Among the SMC complexes, cohesin establishes cohesion between replicated sister chromatids, which forms the basis for faithful chromosome segregation during cell division. A characteristic feature of cohesin is its ability to bind DNA by topological embrace, which underpins sister chromatid cohesion (Haering et al., 2008). The cohesin ring consists of three core components: two SMCs and a kleisin subunit. Mis4Scc2/NIPBL is known as the cohesin loader.

We assembled cohesin onto a linear 125-bp dsDNA substrate in the presence of Mis4-Ssl3 and ADP·BeF3– and separated the gripping reaction by sucrose gradient centrifugation. We visualized this cohesin loading intermediate by cryo-electron microscopy (cryo-EM) at an average resolution of 3.9 Å. The model covers the Psm1 head and proximal coiled coil bound to the Rad21 C terminus, the Psm3 head and neck bound by the Rad21 N-terminal domain, as well as Mis4 and 32 bp of DNA. The DNA lies on top of the engaged ATPase heads, which are nucleotide bound and in a configuration competent for ATP hydrolysis. Mis4 clamps the DNA onto the ATPase heads, making widespread contacts with Psm1 and Psm3. The U-shaped Mis4 hook binds the engaged Psm1-Psm3 ATPase heads, whereas the Mis4 N-terminal handle contacts the Psm3 neck region. Mis4 and Psm3 together form a protein ring that topologically encircles the DNA. The lumen of the ring is lined with positive charges mainly clustered on the Mis4 surface. Although the U-shaped Mis4 hook can be superimposed with a root-mean-square deviation (RMSD) of only 1.0 Å, the angle at which the N-terminal handle emerges is tilted by 40°. The cryo-EM map was of sufficient quality to build amino acids 5–12 of the Rad21 N-tail, forming a loop wedged between the Psm3 ATPase head and the DNA.

> MGRLLRLEVENFKSYRGHQIIGPFEDFTSIIGPNGAGKSNLMDAISFVLGVKSSHLRSTNVKELIYRGKILQRDNTDFTDSSNPTTAYVKLMYELDNGEQREYKRAITPSGATEYKIDEEIVTFSEYCGSLQKENILVRARNFLVFQGDVETIASQSPLELSKLVEQISGSLEYKSEYDKSKDEQDKAVNLSAHSFNKKRGINAELRQYQEQKTEAERYQSQKEKRDSAQLVYLLWKLFHLEKSISSNMAEVTRLKADSIQLIERRDENTKEIEKLKEKEGSIRRNLLAFDRKVRKQEKLIASKRPELISIAEKALESKSNLRKIQRKAAEIEKDYSDQASTLQVLENQLTSLSAAEKEFLKDMQEKEQLKGLRLLPEDKEEYEGLRSEADKLNSNLLFKLQTLNRNIKVTSQSKDSLTSIVGDLESKIKSLHESVSSLDTERADLLAKINEKIESLELEKHDQQKKRLTYSELFHKTQELNEELQSCLQKILEASADRNESKQDAKKREALYALKRIYPEVKGRIIDLCTPTQKKYESAIAAALGKNFDAIVVETQAVAKECIDYIKEQRIGIMTFFPMDTIAASPVNQKFRGTHKGARLAIDVLNFESEYERVMISAVGNTLICDSMTVARDLSYNKRLNAKTVTLEGTVIHKTGLITGGSSNNRSAKHWDDHDFDLLTQTKDRLMHQIGEIEYQKSSCVITESDTVKLHSLESEISLLKDKYTVVSRSVEDKKKEIGHYESLIKEKQPHLSELEMELRNFVKSRDELQIQVEKVEEKIFSGFCKRIGISDIHTYDEIHRTFTQSFTQKQLEFTKQKSLLENRISFEKQRVSDTRLRLERMHKFIEKDQESIDNYEQNREALESEVATAEAELELLKEDFASENSKTEKILLAASEKKLVGKRLVSELTKLSGNITLLESEIDRYVSEWHAILRKCKLEDIDVPLREGSLTSIPIDDVSNSGDITMGEEPSEPVINFEKFGVEVDYDELDEELRNDGSESMASVLQEKLREYSEELDQMSPNLRAIERLETVETRLAKLDEEFAAARKAAKNAKERFNAVKQKRLQKFQAAFSHISEQIDPIYKELTKSPAFPLGGTAYLTLDDLDEPYLGGIKFHAMPPMKRFRDMDQLSGGEKTMAALALLFAIHSYQPSPFFVLDEIDAALDQTNVTKIANYIRQHASSGFQFVVISLKNQLFSKSEALVGIYRDQQENSSRTLSINLEGYVE;> MFYSEAILSKKGPLAKVWLAAHWEKKLSKVQTLHTSIEQSVHAIVTEETAPMALRLSGQLMLGVVRIYSRKARYLLEDCTEALMRLKMSFQPGQVDMIEPATALQSLKGKDAVTQSANLTLPETITEFDLLVPDSTFDFQWSQLLRTPSRSSNTLELHSLPISSSPSFPSSQLSIEAGRNAQVESGFSLGESFAHVGNDMQFHLPISNSGAATPRSVHSDNQSQISIEVGRDAPAAAATDLSGIIGPQMTKSPASSVTHFSTPSMLPIGGTSLDDELLAPVDDLNLDLGLDDLLGDEQGANAPAIEADEQAETSSIHLPSDIMEDDSSRPAAAGVEEGQVVESATAPQQEKINPQKTVRRQRAIIDPVTELSSKQMKKQLADTSSITSPLCLNTSSIVFNATVNFTRNGKFNTSIFSSNLNPKVNELLQADFKQAILRKRKNESPEEVEPAKHQRTDTSTENQETAEVLDPEEIAAAELANITEAAIATLPQETVVQPEGEAPELGSPMGFPVTALESADDSLFDAPPVMLDEADLLGSERLDSSVSEALPSSQTAKDSLRNKWDPYTEGEKVSFQTLSAGCNREEAVQLFFDVLVLATKDVISVKQDVAIQNEITLTAKRGMLLSSL;> MYITKIVIQGFKSYKDYTVIEPLSPHHNVIVGRNGSGKSNFFAAIRFVLSDAYTHLSREERQALLHEGPGATVMSAYVEVTFANADNRFPTGKSEVVLRRTIGLKKDEYSLDKKTVSKTEVINLLESAGFSRSNPYYIVPQGRVTSLTNAKDSERLELLKEVAGTQIYENRRAESNKIMDETIQKSEKIDELLQYIEERLRELEEEKNDLAVYHKKDNERRCLEYAIYSREHDEINSVLDALEQDRIAALERNDDDSGAFIQREERIERIKAEITELNHSLELLRVEKQQNDEDYTNIMKSKVALELQSSQLSRQIEFSKKDESSKLNILSELESKISEKENELSEILPKYNAIVSEADDLNKRIMLLKNQKQSLLDKQSRTSQFTTKKERDEWIRNQLLQINRNINSTKENSDYLKTEYDEMENELKAKLSRKKEIEISLESQGDRMSQLLANITSINERKENLTDKRKSLWREEAKLKSSIENVKDDLSRSEKALGTTMDRNTSNGIRAVKDIAERLKLEGYYGPLCELFKVDNRFKVAVEATAGNSLFHIVVDNDETATQILDVIYKENAGRVTFMPLNKLRPKAVTYPDASDALPLIQYLEFDPKFDAAIKQVFSKTIVCPSIETASQYARSHQLNGITLSGDRSDKKGALTAGYRDYRNSRLDAIKNVKTYQIKFSDLQESLEKCRSEIESFDQKITACLDDLQKAQLSLKQFERDHIPLKDELVTITGETTDLQESMHHKSRMLELVVLELHTLEQQANDLKSELSSEMDELDPKDVEALKSLSGQIENLSHEFDAIIKERAHIEARKTALEYELNTNLYLRRNPLKAEIGSDNRIDESELNSVKRSLLKYENKLQIIKSSSSGLEEQMQRINSEISDKRNELESLEELQHEVATRIEQDAKINERNAAKRSLLLARKKECNEKIKSLGVLPEEAFIKYVSTSSNAIVKKLHKINEALKDYGSVNKKAYEQFNNFTKQRDSLLARREELRRSQESISELTTVLDQRKDEAIERTFKQVAKSFSEIFVKLVPAGRGELVMNRRSELSQSIEQDISMDIDTPSQKSSIDNYTGISIRVSFNSKDDEQLNINQLSGGQKSLCALTLIFAIQRCDPAPFNILDECDANLDAQYRSAIAAMVKEMSKTSQFICTTFRPEMVKVADNFYGVMFNHKVSTVESISKEEAMAFVEG;> MLFEMTPETFKKVNSSNRIIKGLQYTPLASSIPLENGLQNVLYPSSKFQNEPLQLNSEESSIMQRYVDMLNPGATFVNDSETFNFYKNALSAMITEPAMPAMRVNASPVLDQKVCNSDSLSELNDFTKSLIQPSMLMCEPKEKPDASSINTNRSSSDNGFLTPSSSPRSPSCSRVFNAVQLCSPKKSKDDITTPKKRLMEDTYSPRESPSKIQRLQDVLLKQLQDTRLLISQVIEAENSEDFSSNSLFIKREDDDGKHISSHAIEKLYMALTKLSRLGACDKLLEEGSIILVKQILEKELKELPVACYSIINLHDSLTQFPNLDFILKTTALVLFIIFLVPSFKKLQNEESILHLLNILHSIFEYTVPEAIDNIVQSKTSDARTSEIQHLSVLLQKVANVLNILSKVAHEIPLSEAVVIRIVYLFPKVSTLDNSFKTKLPNCNSSSFDFLKAPLFQTLQYLFRLYPYQRDFIIEESLTNFSHLPTARSVSRTYRLSNGKSIQYYSTLFVRLIQSCSIQNLFDSEIVQSESKSTEALHSGNLTEHLKTVESILSKSRHEEYRIANHIVAYLLSRSLKQNKTESDNSFAILTKILLEDLLNMLSLPEWCGTETIIRQFAMNLVMTVTNDKQAVSSKNAALDLISLIVNKVLALFDLSLFEKHNIPAPTNFNDIISFIPSITRLNELSQVSFNHFYFLCKGDISLENILPYNYNKWFSFLLQLRKVCNDSEALKIIDNCIDKNMQKSQEGFQGPSPFKADENDEDIFIISLYHSSLFLNLKFFVSLIIGFLDSPQASLRTKCLRIINQMKTIPSILRTHPEVLAQIISKSNDQSAIVRDTVLDLLGTYIMAYRETIPQIYGCIISGISDPSTIVRKRAIKQLCEVYEATEDLNIRVDIASKLLTRSNDEEETISELSLEVLEKLWFSPASNELDCQKGYEQLTFLEKQKLRVQYFPILKLCAEPSTERHVLLVTSLKTMLTSKEEINLSTLHTQIRLLLSCLFNQLIEVVTEDQVDESTKGILYEIMSTLFVFSRAFPFLFDLSYLHLLKPYLRSASTIEEQRFLYYVVAIFRQVLPFQKEISESFLRSLESVLLQRLTKAGTATLMEIVPCLCSLFTRLNDYERLKKIVVSCLKSLEEARHSENNFQKMVRLIDLIGLFSRYGDLNRINDDWKHSLDFISPECDDAYVILLGYFQKLLKDAKGQLRIHIIDNMSRICLRETSLFISPLMLSTLDMIIAENNVNEVSVLFKSFLELLAADEDLIFEADQKLSLKGKQNVQSNKSVDRDMLKGTKDKQWIEGVSASLMQHFLPCILDSCFSKNLRYSMLGIEILKCIIHQGLVNPRMCFSTIIALESNAIKETREVAILLHTELHRRHESLIDGLYAQSADLIFSLQKTEEYQTFKLGEFSPFQSAYTIVSADKSSKSRKKLIMQILKPLKLDGIDLPSFTEEKVSFVSFCCVCLAGIPYVSIEEPLMIISTVDSVLATIGPTITGWMKKLDHERFKILAGINLCNLIYLKRYIKYAFSISDSSRPIREKKPLTLLNRGYVDLITSDAKPDIVSKLVIKLFEEENILSGEDQVEGEQLTVV> SEISRQEFQRRRQALVEQMQPGSAALIFAAPEVTRSADSEYPYRQNSDFWYFTGFNEPEAVLVLIKSDDTHNHSVLFNRVRDLTAEIWFGRRLGQDAAPEKLGVDRALAFSEINQQLYQLLNGLDVVYHAQGEY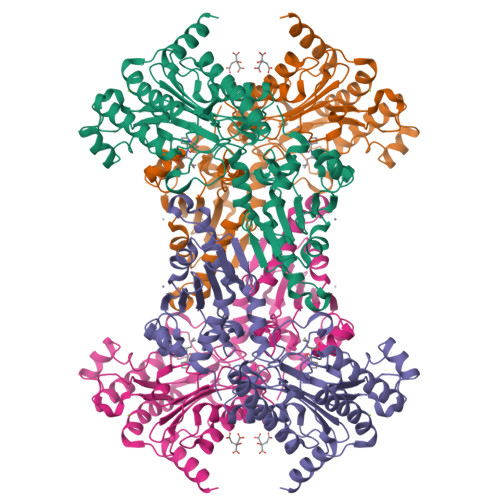AYADVIVNSALEKLRKGSRQNLTAPATMIDWRPVVHEMRLFKSPEEIAVLRRAGEITAMAHTRAMEKCRPGMFEYHLEGEIHHEFNRHGARYPSYNTIVGSGENGCILHYTENECEMRDGDLVLIDAGCEYKGYAGDITRTFPVNGKFTQAQREIYDIVLESLETSLRLYRPGTSILEVTGEVVRIMVSGLVKLGILKGDVDELIAQNAHRPFFMHGLSHWLGLDVHDVGVYGQDRSRILEPGMVLTVEPGLYIAPDAEVPEQYRGIGIRIEDDIVITETGNENLTASVVKKPEEIEALMVAARKQ>MPIHHHHHHQHNLKTSVVESREQRLGTIIAWDGKASDLSKESAYARSEGCGSACGAKARRVCEMRSPFSQGSVCSEQMVECQAGNVRGAVLVQHSPIGCGAGQVIYNSIFRNGLAIRGLPVENLHLISTNLRERDMVYGGLDKLERTIRDAWERHHPQAIFIATSCPTAIIGDDIESVASQLEAEFGIPVIPLHCEGFKSKHWSTGFDATQHGILRQIVRKNPERKQEDLVNVINLWGSDVFGPMLGELGLRVNYVVDLATVEDLAQMSEAAATVGFCYTLSTYMAAALEQEFGVPEVKAPMPYGFAGTDAWLREIARVTHREEQAEAYIAREHARVKPQLEALREKLKGIKGFVSTGSAYAHGMIQVLRELGVTVDGSLVFHHDPVYDSQDPRQDSLAHLVDNYGDVGHFSVGNRQQFQFYGLLQRVKPDFIIIRHNGLAPLASRLGIPAIPLGDEHIAVGYQGILNLGESILDVLAHRKFHEDIAAHVRLPYRQDWLARDPFDLARQSAGQPRRPAE[2x];>MPDAESRSQVTAKAAPPPAPKTNSIEQVRYICSIGAMHSASAIPRVIPITHCGPGCADKQFMNVAFYNGFQGGGYGGGAVVPSTNATEREVVFGGAERLDELIGASLQVLDADLFVVLTGCIPDLVGDDIGSVVGPYQKRGVPIVYAETGGFRGNNFTGH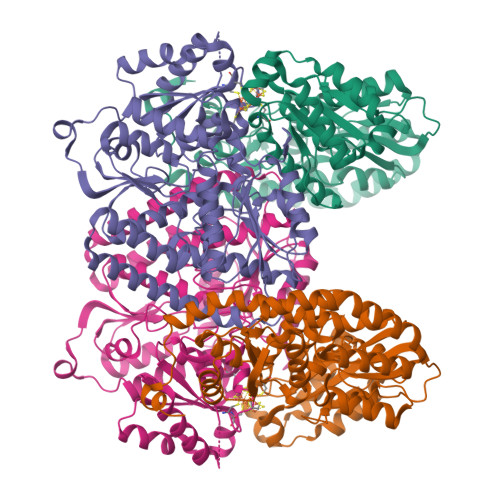ELVTKAIIDQFVGDYDAERDGAREPHTVNVWSLLPYHNTFWRGDLTEIKRLLEGIGLKVNILFGPQSAGVAEWKAIPRAGFNLVLSPWLGLDTARHLDRKYGQPTLHRPIIPIGAKETGAFLREVAAFAGLDSAVVEAFITAEEAVYYRYLEDFTDFYAEYWWGLPAKFAVIGDSAYNLALTKFLVNQLGLIPGLQIITDNPPEEVREDIRAHYHAIADDVATDVSFEEDSYTIHQKIRATDFGHKAPILFGTTWERDLAKELKGAIVEVGFPASYEVVLSRSYLGYRGALTLLEKIYTTTVSASA[2x]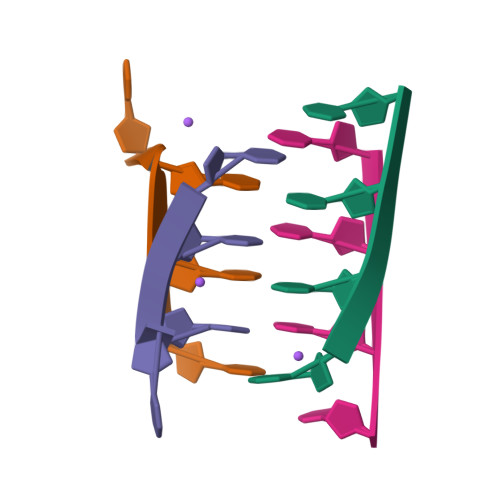>[4x]CCCT> MESLTLQPIARVDGTINLPGSKSVSNRALLLAALAHGKTVLTNLLDSDDVRHMLNALTALGVSYTLSADRTRCEIIGNGGPLHAEGALELFLGNAGIAM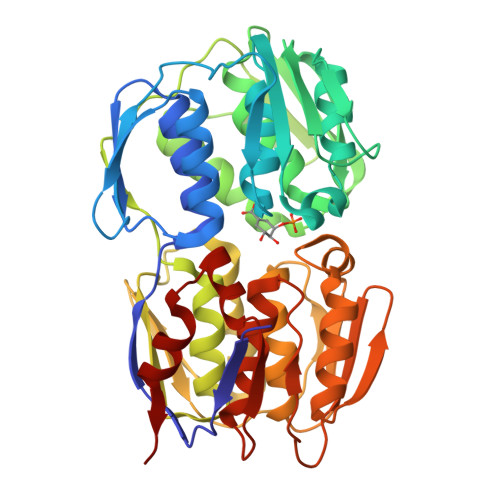RPLAAALCLGSNDIVLTGEPRMKERPIGHLVDALRLGGAKITYLEQENYPPLRLQGGFTGGNVDVDGSVSSQFLTALLMTAPLAPEDTVIRIKGDLVSKPYIDITLNLMKTFGVEIENQHYQQFVVKGGQSYQSPGTYLVEGDASSASYFLAAAAIKGGTVKVTGIGRNSMQGDIRFADVLEKMGATICWGDDYISCTRGELNAIDMDMNHIPDAAMTIATAALFAKGTTTLRNIYNWRVKETDRLFAMATELRKVGAEVEEGHDYIRITPPEKLNFAEIATYNDHRMAMCFSLVALSDTPVTILDPKCTAKTFPDYFEQLARISQAA> MRTTKKIVSAVLAACMLASTAVVSSFAATADDSSAVSSDYARDNSYTKAAEDIDAQYAYSGNDLGVTYTKDATTFKVWSPTATGVKLNIFTKGSDDEQGASKVASYTLEKMLVDGEWNGVWTITLVGEWKDYYYTYSVTTTDTTHIGSDATKTYETQDVYSTATGVNGKRSMIVDLDETDPEGWSNDSHVLLDKSTKSSVWELHIKDFSYDKASGVSDANRGKYLAFTENGTTLNGEGKVSTC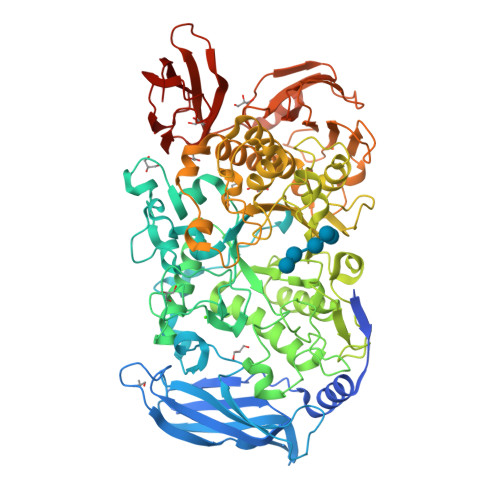IDYLKELGVTTVQLNPFYDFQSVNEAGDDSQFNWGYDPVNYNVPEGSYSSNPYDGKVRIKECKEMIKALHDAGISVVMDVVYNHTYSTDSCFQYTVPNYYYRMKTTGAFSDGSGCGNEGATERAMYRQYVIDSLKYWVNEYHVDGFRFDLMGLMDVETMNMAREALDQIDPRITMWGEGWAGGDSYHPTNTCSGTKFYPATQANASRLSDRIAIFNDGIRDGIKGSAMDISDVGFIQGSKSSAKGVSYGVRANSSGTYKWKAQAPSQCVTYDACHDNATLYDQIIASTGLADYGERNSEAVKMNRLASAIIYTSQGISFTLAGEEMARSKDGDTNSYKSAANLNMIKWQNVVDYADVVSYYKGMMQIKSAFSPLTAMDNSYADKYTFTKKVSASTNQISFTIQNDVEGEWNKMAVIYNNATTAADVTLSDTSVTDWVVIANGETAGLDSLGEVTGSTFTVPARSAIVAVDKAGYESAGIHSSKGKVKVNYVYEATGEKLEDSVILQGSVGSGYVTVPSAVIPDTYIVSRIGGNAEGKYTSDMQEVTYYYTDYIP> GS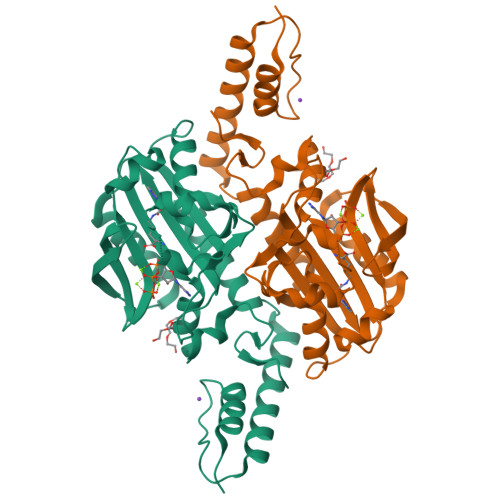HMASAPALTKSQTDRLEVLLNPKDEISLNSGKPFRELESELLSRRKKDLQQIYAEERENYLGKLEREITRFFVDRGFLEIKSPILIPLEYIERMGIDNDTELSKQIFRVDKNFCLRPMLAPNLANYLRKLDRALPDPIKIFEIGPCYRKESDGKEHLEEFTMLNFCQMGSGCTRENLESIITDFLNHLGIDFKIVGDSCMVFGDTLDVMHGDLELSSAVVGPIPLDREWGIDKPWIGAGFGLERLLKVKHDFKNIKRAARSGSYYNGISTNL>[2x]MAKDKEFQVLFVLTILTLISGTIFYSTVE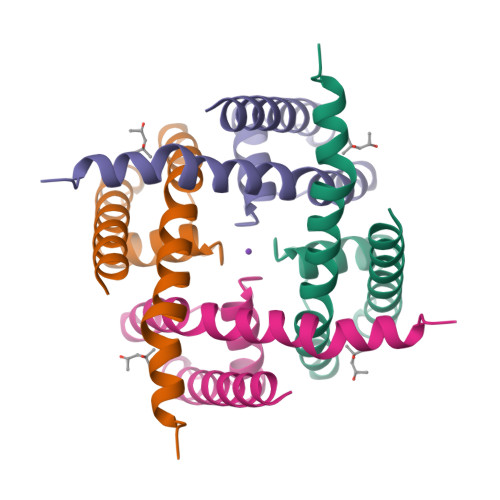GLRPIDALYFSVVTLTTVGYGDFSPQTDFGKIFTILYIFIGIGLVFGFIHKLAVNVQLPSILSNLVPR> MGSSHHHHHHSQDPQDLNFGQVVADVLCEFLEVAVHLILYVREVYPVGIFQKRKKYNVPVQMSCHPELNQYIQDTLHCVKPLLEKNDVE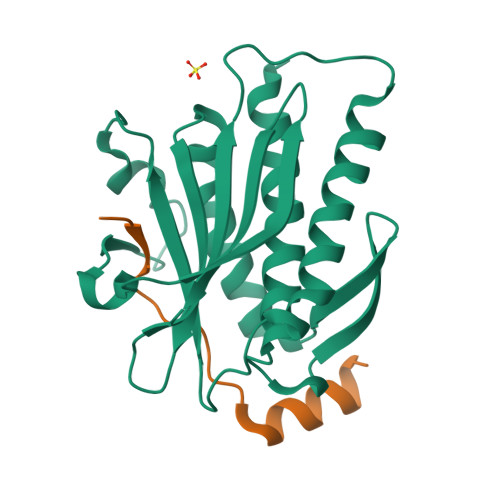KVVVVILDKEHRPVEKFVFEITQPPLLSISSDSLLSHVEQLLAAFILKISVCDDVLDHNPPGCTFTVLVHTREAATRNMEKIQVIKDFPWILADEQDVHMHDPRLIPLKTMTSDILKMQLYVEERAHKGS;> MGSKLPLRPKRSPPVISEEAAEDVKQYLTI>MISRIMLHKNTLLFAALSAALWGGATQAANAAVVASLKPLGFIASAIADGVTDTQVLLPDGASEHDYSLRPSDVKRLQGADLVVWIGPEMEAFMEKSVKNIPDGKQVTIAQLADVKPLLMKGADDDHDHGHEHGEKGDAHHHHGDYNMHLWLSPEIARASAVAIHEKLVELMPQSRAKLDANLKDFEAQLAATDKQVGNELAPLKGKGYFVFHDAYGYYEKHYGLTPLGHFTVNPEIQPGAQRLHEIRTQLVEQKATCVFAEPQFRPAVVEAVARGTSVRMGTLDPLGTNIKLGKTSYSAFLNQLANQYASCLKGD[6x]

In bacteria, high-affinity zinc import is accomplished by ATP-binding cassette (ABC) transporters, which rely on extracellular solute-binding proteins (SBPs) to acquire the metal and deliver it to the membrane permease. By this classification, SBPs that bind zinc, manganese or iron belong to cluster A-I, which is defined by two related α/β domains linked by a long α-helix. The ZnuA proteins of Gram-negative species primarily belong to group II, which is defined by zinc specificity, the presence of a long flexible loop rich in His and Asp/Glu residues, and metal coordination by three His residues and one Glu residue or water in a tetrahedral geometry. Here, we characterize zinc binding to the cluster A-I SBP ZnuA from the human pathogen Citrobacter koseri (Ck ZnuA) and present the crystal structure of the holo form.

A screen of additives identified hexatungstotellurate (TEW; Mauracher et al., 2014) to contribute to larger, better-ordered crystals, as has previously been reviewed. These crystals belonged to space group P2, with six copies of Ck ZnuA in the asymmetric unit. With a formal charge of minus six, TEW often interacts electrostatically with positively charged residues and through hydrogen bonding in protein structures. Each TEW in the Ck ZnuA structure is in close proximity to Lys91 of four symmetry-related protein chains. All residues could be modeled into the electron density with the exception of the His-rich loop, which is typical of cluster A-I SBP structures, where this region is disordered. In all six chains zinc is bound between the domains and is coordinated by Glu59, His60, His147 and His211.>[4x]GGGHMIKNCKILNLRAIRDNRGSLIALENNKEVPFEIKRVYYIFDTDPNFPRGAHAHKNLEQVLIMMSGSCDIILNDGKNYEKICLNRPDIGLYIGKNMWREMKNFSYGAKLLVLASDFY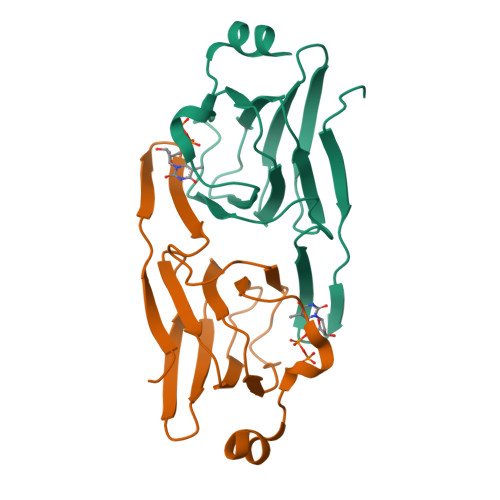DAAAYIRNYDEFLRNINDT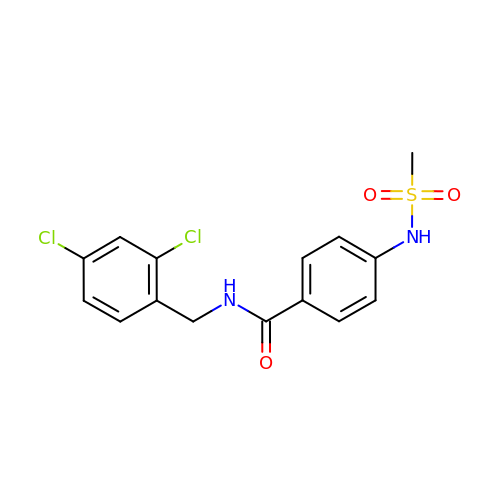N-[(2,4-dichlorophenyl)methyl]-4-[(methylsulfonyl)amino]benzamide | C15 H14 Cl2 N2 O3 S | RDFIQTZRJRVFHK-UHFFFAOYSA-N> SNAMDAETDRAEIIELFGRYADIADLKEFTDLPRRVHTDPLT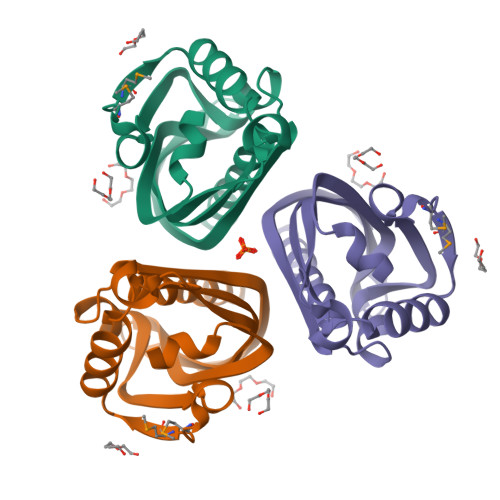IDFESVTGMPPMTVPLSDYGAALRASFGAFSATHHAITGHVVTIDSDRATIHAHVRAEHWLPAEVAGDGPDRWLVVGFYDNEAVRTADGWRLSSVKLTASYQENAHLARAAAAGQAG> MSFVSKLLYTVSALVLFHSGFSSYEFHHLLKLNSLNNAQGAISKLPKDIMYET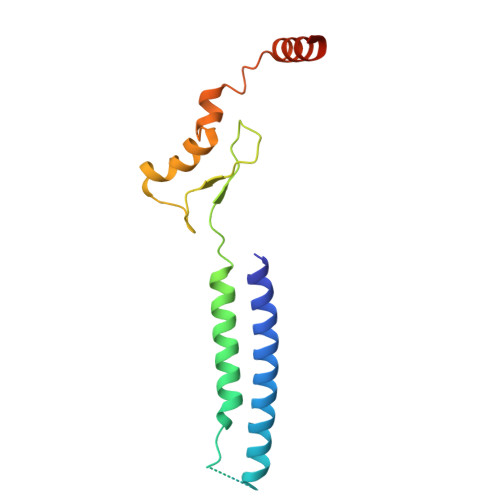YAGLILFVLAVFTSFEKLQYLPIESNDGKIISQGNYLKEIALNKATNVDNLIGSNPNGEIIFTPSFVDVHMKRKICREWASNTVKKEK>MAHHHHHHMLKVIVETKTLVQALGFASSVVEKRNIISELANIKLLAKDGLLELSSTNMDLYLSQKIGVQVVSEGELTVSTKTLNDIVKKLPDSELTLTDLGTTGLEITGKNCRFNLFTLPVESFPVMDNINPEASFKISCAEFAKIIESTKFSVSLDETRYNLNGIYLHVKDSEFYAASTDGHRLSVSSVVLAEKIEDFGVILPQKSAEEILKIVKDSKNANADIEILLSSNKIKFICN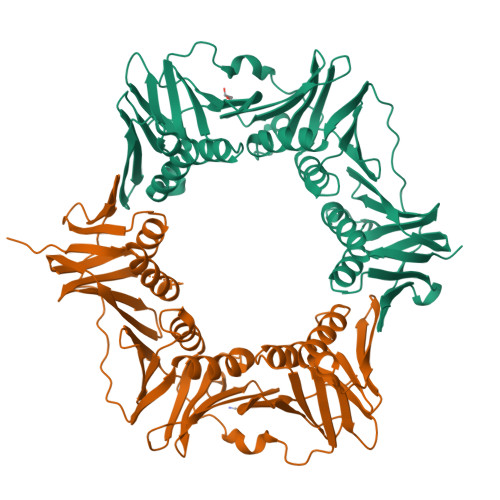ENVIMLSKLIDGTFPDYSSFIPENSSSKLVINRKIFADTIERIAIITVEKFRAVKLSLSGEALEISAIGEARGNAKEVINSSKETENFYEYSGETNLDIGFNPQYLEDVLKAIKSDLVELYFSSVSAPVLIKFPESPKDIFVVMPVKV[2x]>MKQYLELMQKVLDEGTQKNDRTGTGTLSIFGHQMRFNLQDGFPLVTTKRCHLRSIIHELLWFLQGDTNIAYLHENNVTIWDEWADENGDLGPVYGKQWRAWPTPDGRHIDQITTVLNQLKNDPDSRRIIVSAWNVGELDKMALAPCHAFFQFYVADGKLS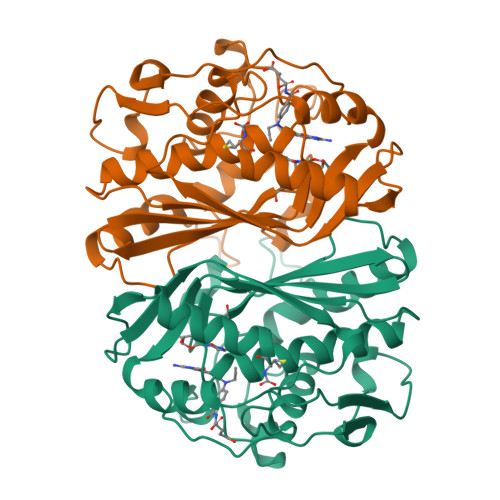CQLYQRSCNVFLGLPFNIASYALLVHMMAQQCDLEVGDFVWTGGDTHLYSNHMDQTHLQLSREPRPLPKLIIKRKPESIFDYRFEDFEIEGYDPHPGIKAPVAI[2x]>TEFSEEQKRTLDLLFLFDRRMTEERRRWLSQRLGLNEEQIERWFRRKEQQI[4x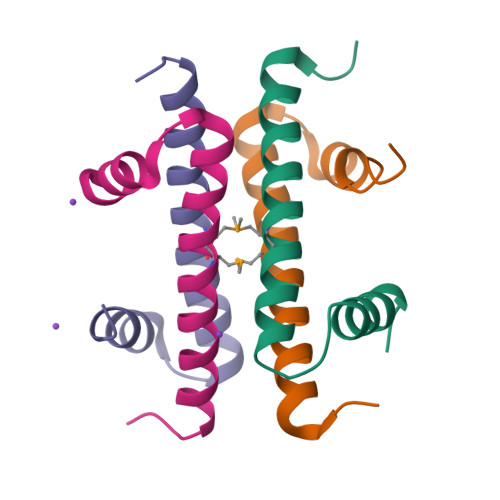]> GPAMAGKSIPFPLKDIKSVVEVFRQELRNDQPNLAQLSIVLGFFESASTMKAGDTTSTPSLDEETFDALHCKFMALLQRDFTFNAGGLPATREIVKNVADLVWGCLAKSYFKDRPHIQNLYSFLTGNRLDCFGVAFAVVAMCQALGYNDVHLALSEDHAWVVFGKDKIETAEVTWHGKGNEDKRGKPVIYQDDDRCSWLYLNGN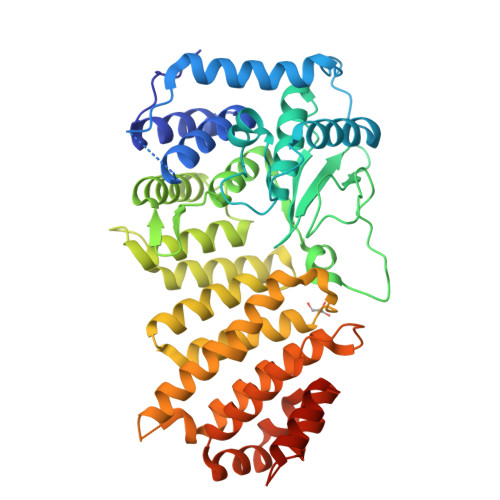AVHCTRHMEVASIISSINPNINHTTDSIQLSQLQQELLWLLYDMGHIKTYPMAIANLGDLEEISPTPGRPPAEELFKEAITVAKREYSDHHIYPYTYLGGYYYRKKKYYEAIASWVDAGYVAGKYNYSKDDEEMYKEFHEIANDLIPNILKDAVAKADPSGTGSTNLTSDPKFFALVLQFYDGICLWEEGSPTPVLHADWAKKLVQSIGKFAPECRSAFNANTDTLSLRSAKMREMKNLITTSGKLNTSAMKLQLTAQSQVNVPKSRR> RNDRTLRRMRKVVNIINAMEPEMEKLSDEELKGKTAEFRARLEKGEVLENLIPEAFAVVREASKRVFGMRHFDVQLLGGMVLNERCIAEMRTGEGKTLTATLPAYLNALTGKGVHVVTVNDYLAQRDAENNRPLFEFLGLTVGINLPGMPAPAKREAYAADITYGTNNEYGFDYLRDNM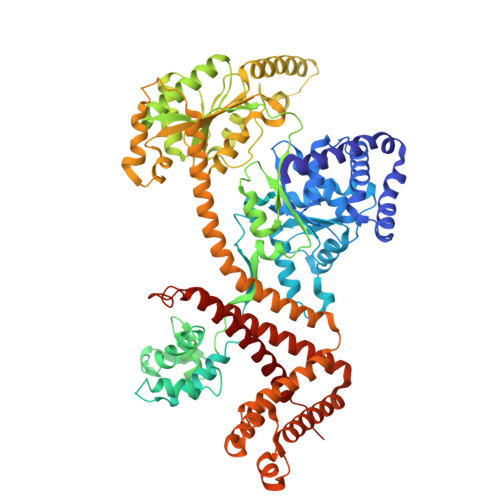AFSPEERVQRKLHYALVDEVDSILIDEARTPLIISGPAEDSSEMYKRVNKIIPHLIRQEKEDSETFQGEGHFSVDEKSRQVNLTERGLVLIEELLVKEGIMDEGESLYSPANIMLMHHVTAALRAHALFTRDVDYIVKDGEVIIVDEHTGRTMQGRRWSDGLHQAVEAKEGVQIQNENQTLASITFQNYFRLYEKLAGMTGTADTEAFEFSSIYKLDTVVVPTNRPMIRKDLPDLVYMTEAEKIQAIIEDIKERTAKGQPVLVGTISIEKSELVSNELTKAGIKHNVLNAKFHANEAAIVAQAGYPAAVTIATNMAGRGTDIVLGGSWQAEVAALENPTAEQIEKIKADWQVRHDAVLEAGGLHIIGTERHESRRIDNQLRGRSGRQGDAGSSRFYLSMEDALMRIFASDRVSGMMRKLGMKPGEAIEHPWVTKAIANAQRKVESRNFDIRKQLLEYDDVANDQRRAIYSQRNELLDVSDVSETINSIREDVFKATIDAYIPPQSLEEMWDIPGLQERLKNDFDLDLPIAEWLDKEPELHEETLRERILAQSIEVYQRKEEVVGAEMMRHFEKGVMLQTLDSLWKEHLAAMDYLRQGIHLRGYAQKDPKQEYKRESFSMFAAMLESLKYEVISTLSKVQVRMP> MGLFDRLGRVVRANLNDLVSKAEDPEKVLEQAVIDMQEDLVQLRQAVARTIAEEKRTEQRLNQDTQEAKKWEDRAKLALTNGEENLAREALARKKSLTDTAAAYQTQLAQQRTMSENLRRNLAALEAKISEAKTKKNMLQARAKAAKANAELQQTLAAAAAA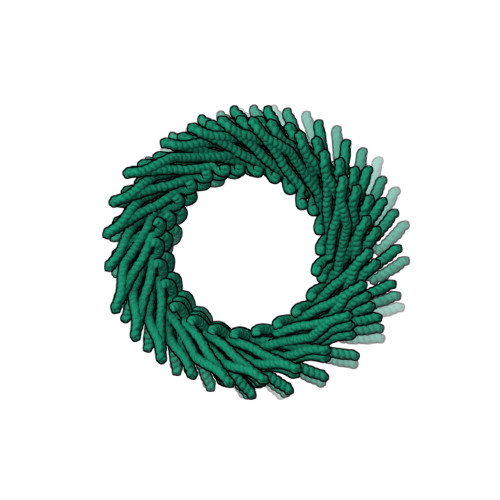AAAAAFERMENKVLDMEATSQAAGELAGFGIENQFAQLEASSGVEDELAALKASMAGGALPGTSAATPQLEAAPVDSSVPANNASQDDAVIDQELDDLRRRLNNLAALEVLFQGP> LSTCTTLDFGHIKKKRVEAIRGQILSKLRLTSPPEPTVMTHVPYQVLALYNSTRELLEEMHGEREEGCTQENTESEYYAKEIHKFDMIQGLAEHNELAVCPKGITSKVFRFNVSSVEKNRTNLFRAEFRVLRVPNPSSKRNEQRIELFQILRPDEHIAKQRYIGGKNLPTRGTAEWLSFDVTDTVREWLLRRESNLGLEISI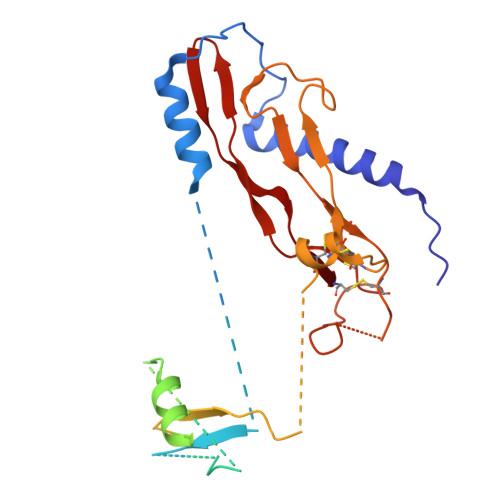HCPCHTFQPNGDILENIHEVMEIKFKGVDNEDDHGRGDLGRLKKQKDHHNPHLILMMIPPHRLDNPGQGGQRKKRALDTNYCFRNLEENCCVRPLYIDFRQDLGWKWVHEPKGYYANFCSGPCPYLRSADTTHSTVLGLYNTLNPEASASPCCVPQDLEPLTILYYVGRTPKVEQLSNMVVKSCKCS> XGPKGPPGDKGPPGDPGPPGARGEPGN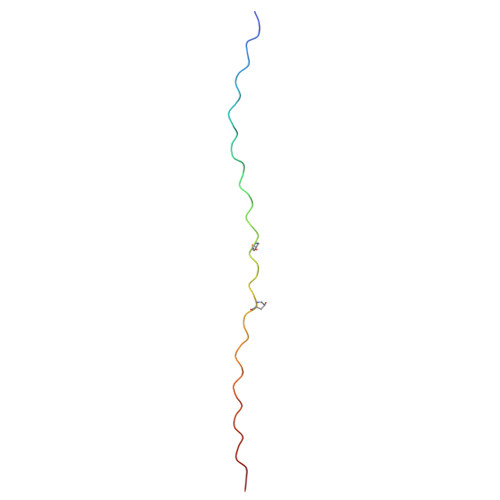IGFPGPPGPKGPKGDPGDPGGY>MQKPVCLVVAMTPKRGIGINNGLPWPHLTTDFKHFSRVTKTTPEEASRLNGWLPRKFAKTGDSGLPSPSVGK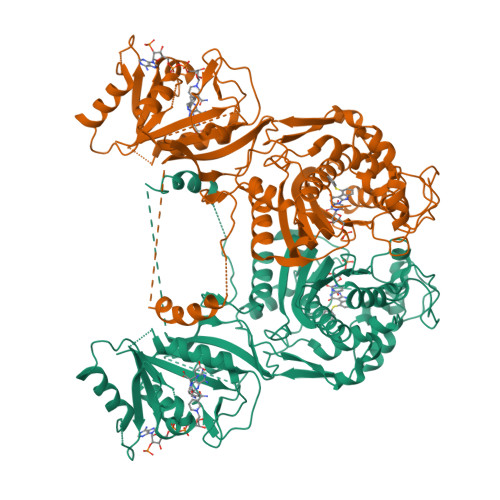RFNAVVMGRKTWESMPRKFRPLVDRLNIVVSSSLKEEDIAAEKPQAEGQQRVRVCASLPAALSLLEEEYKDSVDQIFVVGGAGLYEAALSLGVASHLYITRVAREFPCDVFFPAFPGDDILSNKSTAAQAAAPAESVFVPFCPELGREKDNEATYRPIFISKTFSDNGVPYDFVVLEKRRKTDDAATAEPSNAMSSLTSTRETTPVHGLQAPSSAAAIAPVLAWMDEEDRKKREQKELIRAVPHVHFRGHEEFQYLDLIADIINNGRTMDDRTGVGVISKFGCTMRYSLDQAFPLLTTKRVFWKGVLEELLWFIRGDTNANHLSEKGVKIWDKNVTREFLDSRNLPHREVGDIGPGYGFQWRHFGAAYKDMHTDYTGQGVDQLKNVIQMLRTNPTDRRMLMTAWNPAALDEMALPPCHLLCQFYVNDQKELSCIMYQRSCDVGLGVPFNIASYSLLTLMVAHVCNLKPKEFIHFMGNTHVYTNHVEALKEQLRREPRPFPIVNILNKERIKEIDDFTAEDFEVVGYVPHGRIQMEMAV[8x]>MWVLLRSGYPLRILLPLRGEWMGRRGLPRNLAPGPPRRRYRKETLQALDMPVLPVTATEIRQYLRGHGIPFQDGHSCLRALSPFAESSQLKGQTGVTTSFSLFIDKTTGHFLCMTSLAEGSWEDFQASVEGRGDGAREGFLLSKAPEFEDSEEVRRIWNRAIPLWELPDQEEVQLADTMFGLTKVTDDTLKRFSVRYLRPARSLVFPWFSPGGSGLRGLKLLEAKCQGDGVSYEETTIPRPSAYHNLFGLPLISRRDAEVVLTSRELDSLALNQSTGLPTLTLPRGTTCLPPALLPYLEQFRRIVFWLGDDLRSLEAAKLFARKLNPKRCFLVRPGDQQPRPLEALNGGFNLSRILRTALPAWHKSIVSFRQLREEVLGELSNVEQAAGLRWSRFPDLNRILKGHRKGELTVFTGPTGSGKTTFISEYALDLCSQGVNTLWGSFEISNVRLARVMLTQFAEGRLEDQLDKYDHWADRF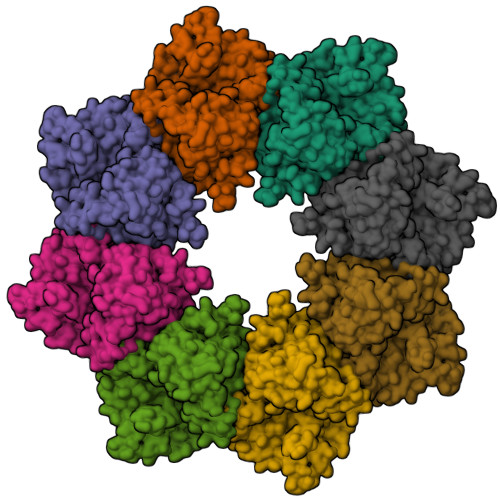EDLPLYFMTFHGQQSIRTVIDTMQHAVYVYDICHVIIDNLQFMMGHEQLSTDRIAAQDYIIGVFRKFATDNNCHVTLVIHPRKEDDDKELQTASIFGSAKASQEADNVLILQDRKLVTGPGKRYLQVSKNRFDGDVGVFPLEFNKNSLTFSIPPKNKARLKKIKDDTGPVAKKPSSGKKGATTQNSEICSGQAPTPDQPDTSKRSKAAALEHHHHHH[8x]Birt–Hogg–Dubé syndrome (BHD) is an inherited genetic disorder that predisposes individuals to renal cell carcinoma (RCC), benign skin tumours and lung cysts that lead to recurrent spontaneous pneumothorax. In BHD patients, the most common germline mutation that can lead to RCCs occurs in the mutation hotspot, exon 11, of the FLCN gene, and produces a truncated folliculin protein that lacks the C-terminal half. In this study, we use structural and biochemical analyses to show that folliculin is probably a distant relative of the differentially expressed in normal cells and neoplasia (DENN) family of guanine nucleotide exchange factors (GEFs) and demonstrate that it possesses in vitro nucleotide exchange activity towards Rab35 GTPase. Through structure–function analyses, we report that folliculin, which is commonly mutated in patients suffering from these malignancies, has an unusual architecture that classes it into an ancient family of proteins called the DENNs.

In order to understand the essentiality of the C-terminal region (amino acids 341–566) and reveal the function of full-length folliculin, we have determined at 2 Å resolution the three-dimensional structure of the C-terminal domain of folliculin, henceforth called folliculin-CT. We have calculated phases by the multi-wavelength anomalous dispersion (MAD) method using anomalous scatterers from selenomethionine (see §4). The folliculin-CT crystallized in C2221 space group with two molecules in the asymmetric unit related by twofold non-crystallographic symmetry. The fold of folliculin-CT is dominated by an αβ architecture with a core β-sheet and helices packed on the one side, followed by an all-helical region. Indeed, the strand topology differs, and the signature Walker A and B motifs conserved for function across NTPase families are absent in the folliculin-CT domain. Interestingly, folliculin-CT shares remarkable structural similarity with the DENN domain of the DENN1B-S protein; both proteins have the same order and orientation of strands. Although the sequence identity is only 11 per cent, a structural alignment using the program Baton (based on Comparer) shows a r.m.s.d. of 2.8 Å over its 170 core-aligned residues, corroborating the strong similarity and probable homology. Indeed, biochemical analysis of a representative set of Rabs reveals that folliculin-CT, in vitro, has GEF activity towards Rab35, and this is confirmed using a subset of Rabs with the full-length folliculin, which shows similar activity to the folliculin-CT. The truncated folliculin polypeptide chain found in BHD syndrome is missing the c-DENN and d-DENN modules, and retains only the u-DENN region—which is the only part of the DENN homology region that is kept in the more compact yeast folliculin orthologue, LST7.

>RKLPVFKSLRHMRQVLGAPSFRMLAWHVLMGNQVIWKSRDVDLVQSAFEVLRTMLPVGCVRIIPYSSQYEEAYRCNFLGLSPHVQIPPHVLSSEFAVIVEVHAAARSTLHPVGAEDDQSLSKYEFVVTSGSPVAADRVGPTILNKIEAALTNQNLSVDVVDQALVALKEEWMNKVKVLFKFTKVDSRPKEDTQKLLSILGASEEDNVKLLKFWMTGLSKTYKSHLM[2x]> TSFAEY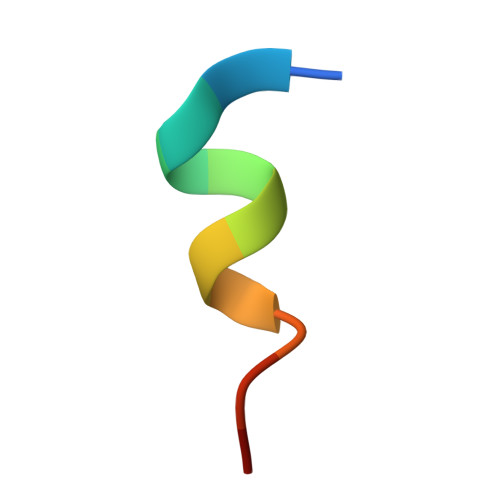WNLLSP> GSEPCVEVVPNITYQCMELNFYKIPDNLPFSTKNLDLSWNPLRHLGSYSFFSFPELQVLDLSRCEIQTIEDGAYQSLSHLSTLILTGNPIQSLALGAFSGLSSLQKLVAVETNLASLENFPIGH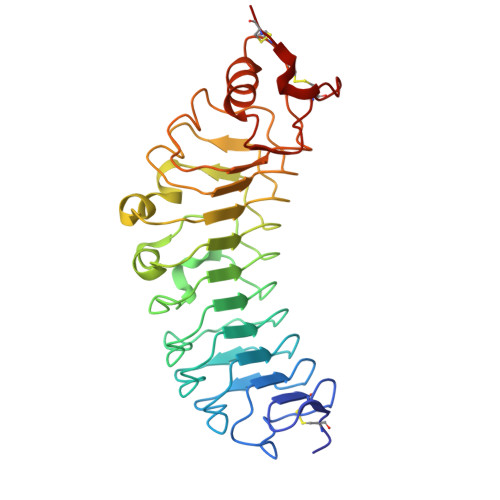LKTLKELNVAHNLIQSFKLPEYFSNLTNLEHLDLSSNKIQSIYCTDLRVLHQMPLLNLSLDLSLNPMNFIQPGAFKEIRLKELALDTNQLKSVPDGIFDRLTSLQKIWLHTNPWDCSCPRIDYLSRWLNKNSQKEQGSAKCSGSGKPVRSIICPT ALDOSTERONE | C21 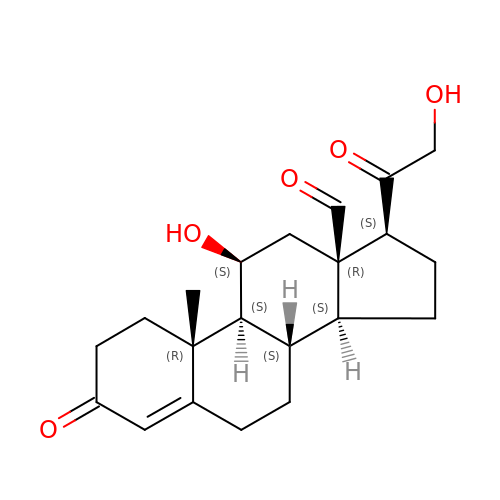H28 O5 | PQSUYGKTWSAVDQ-ZVIOFETBSA-N Under conditions of sulphur limitation and in the presence of the inducer, N-acetylserine, CysB binds to cys promoters and activates the transcription of the downstream coding sequences. CysB is a homotetramer of 36 kDa subunits, each comprising a smaller N-terminal DNA binding domain and a C-terminal effector binding domain. CysB is a member of the LysR-type transcriptional regulator (LTTR) family, named after its founding member. To elucidate the subunit arrangement in the tetramer, we determined the crystal structure of intact CysB in complex with N-acetylserine.

The H32 and H3 crystal structures have 2 and 8 molecules in the asymmetric unit respectively. In the H32 crystal form, a crystallographic twofold axis of symmetry generates the CysB tetramer while the asymmetric unit of the H3 crystal form contains two CysB tetramers. There are two protomer types in each tetramer distinguished by the juxtaposition of the DNA binding and the effector binding domains. In each tetramer, two of the chains (B and D) adopt the extended conformation as illustrated for Molecule B in Fig. 1A while the other two chains (A and C) exhibit a compact conformation as shown for Molecule A in Fig. 1B. The change in overall structure arises from alternative conformations of hinge regions flanking the linker helix. In the tetramer as shown in Fig. 1D, the four effector binding domains form a core from which the DNA binding domains project in pairwise arrangements, A-D and B-C. The interface between subunits A and B is extensive at 1540 Å2 with 45 residues on each chain participating. The interactions between chains A and D, equivalent to those between chains C and B, are dominated by the packing of the linker helices. To investigate potential larger scale structural changes, we performed a normal mode analysis of the N-acetylserine bound ABCD CysB tetramer in the H3 crystal form using the tools available at WEBnm@. In the lowest frequency mode, the origin of motion appears to be at the twofold axis running through the core of the tetramer resulting in modest movements of the EBDs of chains A and C and larger movements of the EBDs of chains B and D. These movements radiate out to the DNA binding domains with the largest movements occurring at DBDB and DBDD which are furthest from the two-fold axis.

>[8x]MKLQQLRYIVEVVNHNLNVSSTAEGLYTSQPGISKQVRMLEDELGIQIFARSGKHLTQVTPAGQEIIRIAREVLSKVDAIKSVAGEHTWPDKGSLYVATTHTQARYALPGVIKGFIERYPRVSLHMHQGSPTQIAEAVSKGNADFAIATEALHLYDDLVMLPCYHWNRSIVVTPEHPLATKGSVSIEELAQYPLVTYTFGFTGRSELDTAFNRAGLTPRIVFTATDADVIKTYVRLGLGVGVIASMAVDPVSDPDLVKLDANGIFSHSTTKIGFRRSTFLRSYMYDFIQRFAPHLTRDVVDTAVALRSNEDIEAMFKDIKLPEK> MHHHHHHITSLYKK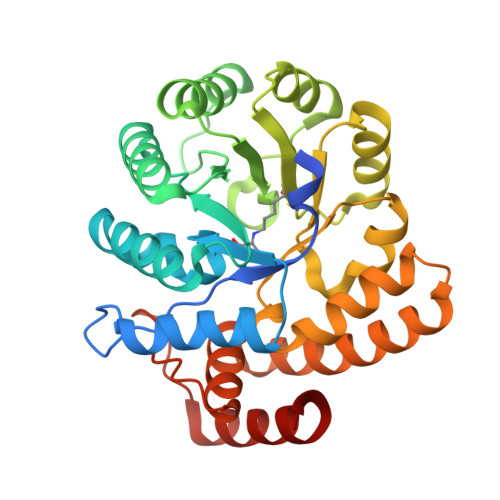AGFMKGIYSALMVPYNEDGSINEKGLREIIRYNIDKMKVDGLYVGGSTGENFMISTEEKKRVFEIAIDEAKDSVNLIAQVGSINLNEAVELGKYVTKLGYKCLSAVTPFYYKFDFSEIKDYYETIVRETGNYMIIYSIPFLTGVNMSLSQFGELFENEKIIGVKFTAGDFYLLERVRKAFPDKLIFAGFDEMLLPATVLGVDGAIGSTYNINGIRAKQIFELAKNSKIDEALKIQHTTNDLIEGILSNGLYQTIKEILKLEGVDAGYCRKPMKKISQKQIEFAKELHKKFLKN> MSS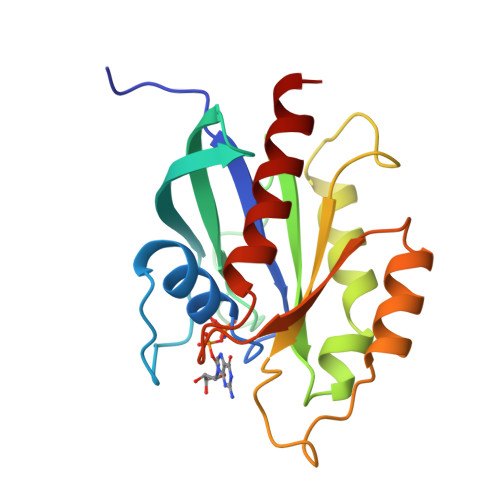RKKNILKVIILGDSGVGKTSLMHRYVNDKYSQQYKATIGADFLTKEVTVDGDKVATMQVWDTAGQERFQSLGVAFYRGADCCVLVYDVTNASSFENIKSWRDEFLVHANVNSPETFPFVILGNKIDAEESKKIVSEKSAQELAKSLGDIPLFLTSAKNAINVDTAFEEIARSALQQNQA4-(imidazol-1-ylmethyl)-3-(4-methoxyphenyl)-1-phenyl-pyrazole 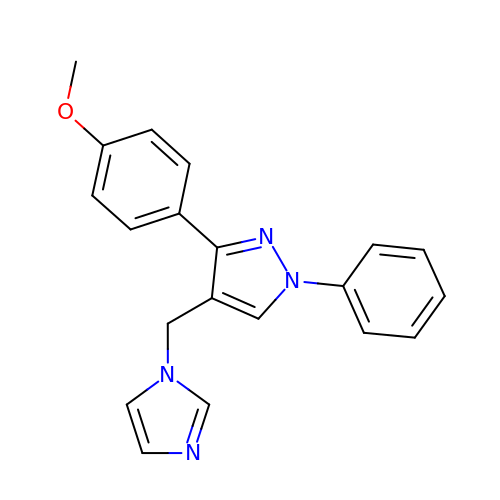| C20 H18 N4 O | CZOCKHTYPCJURT-UHFFFAOYSA-N> 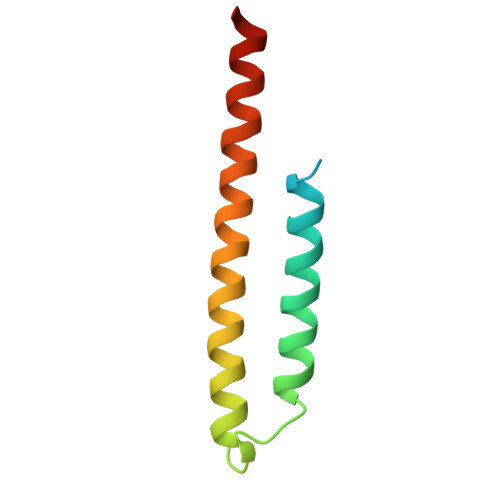TNKYHEKWISKFAPGNELSKKYLAKVKERHELKEFNNSISAQDNYAKWTKNNRKLDSLDKEINNLKDEIQSENKAFQAHLHKLR>EMKPHPWFFGKIPRAKAEEMLSKQRHDGAFLIRESESAPGDFSLSVKFGNDVQHFKVLRDGAGKYFLGV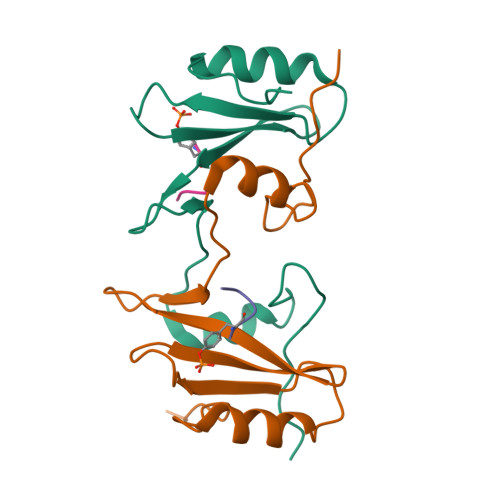VKFNSLNELVDYHRSTSVSRNQQIFLRDIEQ[16x];>SYVNVQ[16x]>MASMTGGQQMGRGSMAPTTPNGGKPSQDLTLVGAASGPVALHNVAPGTASTDAVNVGQLGAVTTGLGGGAAIDPKTGAVTAPSYTVYNADGTTSNVGNVGAAIDAINSTGIKYFHANSTKPDSQALGADSVAIGPNAVANNAGDVALGSGAVTSQAGGTLSETINGVTYSFAGTTPIGTVSVGAPGVERTITNVAAGRIGQSSTDAINGSQLYGTNQSIEALTDKMNSLGNTVANTLGSGASYNPQTGAVNGPANSGGVVTPTVIQEAANKWVSANPSTYVAPVATGTNGMAVGSGAVSTGQNSVALGTNASDGGRSN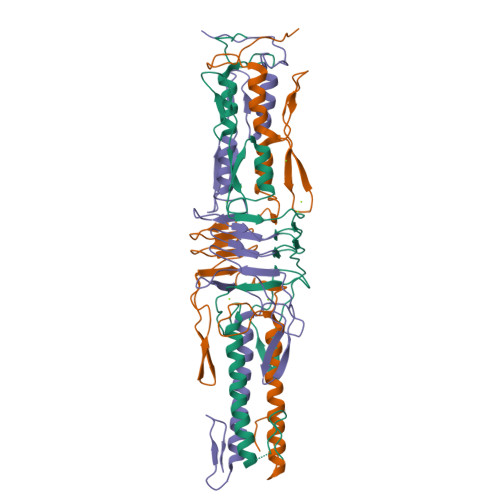VVSVGAPGAERQVTNVAAGTQATDAVNLGQMNGANSSSVDKLAAALEHHHHHH[3x]> GMQMELQSPEYKLSKLRTSTIMTDYNPNYCFAGKTSSISDLKEVPRKNITLIRGLGHGAFGEVYEGQVSGMPNDPSPLQVAVKTLPEVCSEQDELDFLMEALIISKFNHQNIVRCIGVSLQSLPRFILLELMAGGDLKSFLRETRPRPSQPSSLAMLDLLHVARDIACGCQYLEENHFIHRDIAARNCLLTCPGPGRVAKIGDFGMARDIYRASYYRKGGCAMLPVKWMPPEAFMEGIFTSKTDTWSFGVLLWEIFSLGYMPYPSKSNQEVLEFVTSGGRMDPPKNCPGPVYRIMTQCWQHQPEDRPN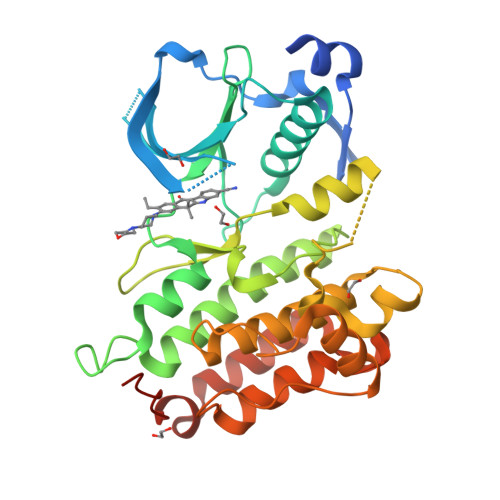FAIILERIEYCTQDPDVINTALPIEYGPLVEEEEKV> MIVGGSTIQPERVDAAALRQLGDAMRKVVGSADPTPLADLLSGTPVDPDELTREVGADGRQALLDSGMAVDDGTTFSSPLRGHQLHGVVVLSDPDVEEEVQHRWYVDPLWEADLLIRLMLRRGGARALDMGCGSGVLSLVLADRYESVLGVDVNPRAVALSRLNAALNGLTNVTFREGDMFEPAEGRFSRIVFNSPTNEEGNEFVDLLEAGEPILETFFRNVPR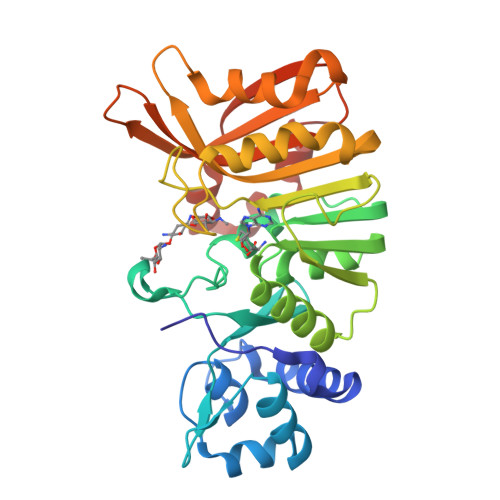KLESGGIVEVNLAMNDYPGDPFRERLADWLGLTENGLRVQIFTSQRRATESGGEWKRGWLVVAPGPVGLTEVEWPYHDRYEEDPDALLDGTDRLLRG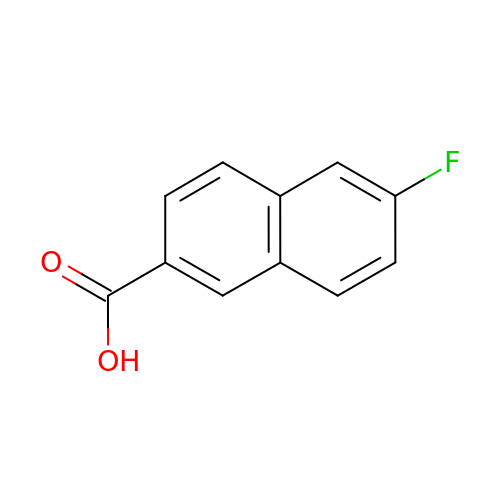6-fluoranylnaphthalene-2-carboxylic acid | C11 H7 F O2 | CYKDCZRPLWJEKA-UHFFFAOYSA-N(2~{R})-2-[[(2~{R})-5-chloranyl-1-methyl-2,3-dihydroindol-2-yl]carbonylamino]-2-cyclohexyl-ethanoic 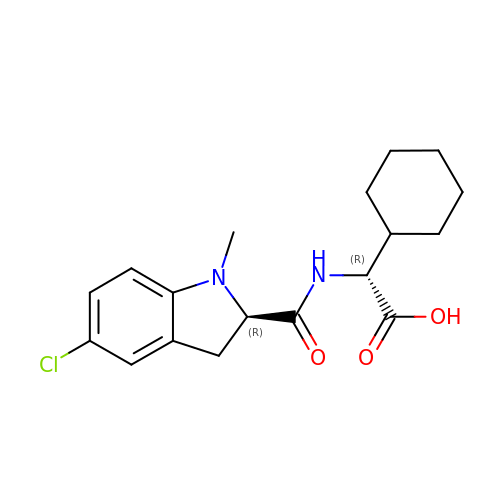acid | C18 H23 Cl N2 O3 | CURRXVCCZQBGQB-HZPDHXFCSA-N>MLSHMVLTRQDIGRAASFYEDGADDYYAKDGDASEWQGKGAEELGLSGEVDSKRFRELLAGNIGEGHRIMRSA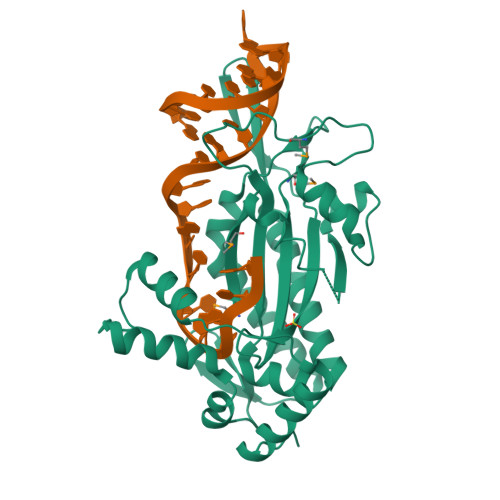TRQDSKERIGLDLTFSAPKSVSLQALVAGDAEIIKAHDRAVARTLEQAEARAQARQKIQGKTRIETTGNLVIGKFRHETSRERDPQLHTHAVILNMTKRSDGQWRALKNDEIVKATRYLGAVYNAELAHELQKLGYQLRYGKDGNFDLAHIDRQQIEGFSKRTEQIAEWYAARGLDPNSVSLEQKQAAKVLSRAKKTSVDREALRAEWQATAKELGIDFS[2x]> DDVVTFKAQEQLQRASEQAHNSPVLRALLAESLRLFEQVAGSLTPANLTTAVEQYISLKYYAGAIQLCLTVAQQKDRGNTALSWVNDGKPANDSRKKAFDERKICYNLIHQVLDKLESDFAGEPELVDGRPTLAATKRMEAYNVVNDSSDEVFHFDLYEWYIEKGWTDRILSIDSPHVITYLQRLAETDFRHAELLCRFYTTRSRFFEAAQVQTNLAKSDLNISLKDRIILLSRAKGNASVNTIGISRQQQQQLNHEASELLEIAHIQDDLLERLVADPRIPEERKAEIEEFLDGPIRTLTDLFNDYADQANYYDLCLLIFHAADFHNPRTILDTWNNLINQSHFEAEQRREYWEIVQAGGDLPAGVIAPIAEPPLPYVYVSQQIQLIAHRTSLDSLIFPVNSLLPVVCAYAINNGQDASIGADPCWPIQLFLNLGVPHALVVQVLENVLDTQEAPFTGRRRKLVVQWIAMAVDMWVREVERRGAMAAAAASGASGSEAVMGSWVSELLGRADQVLTQIAGTGAGGAASDAEEIASLRRTVKGL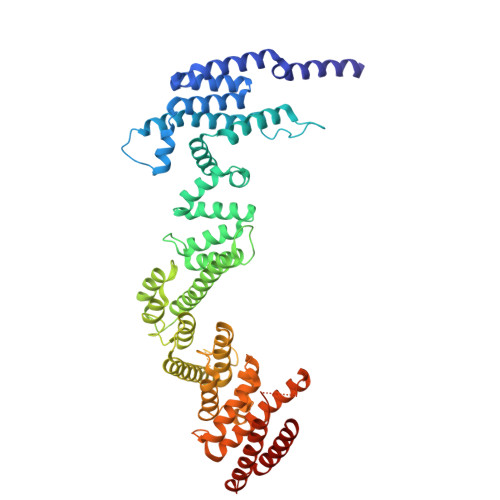KRSVD ZCCHC4 is a newly identified m6A RNA methyltransferase and is highly conserved in multicellular organisms. ZCCHC4-mediated m6A4220 methylation in 28S rRNA promotes ribosome assembly and translation, which in turn impacts cell proliferation and tumor growth. Distinct from what was observed for all other m6A methyltransferases, ZCCHC4 is organized into four domains, with three flanking zinc finger domains packed around the MTase domain, forming an integrated RNA-binding platform. Through structural, biochemical, and enzymatic characterization of ZCCHC4, a recently reported rRNA m6A writer, this study reveals the molecular basis for the ZCCHC4-mediated m6A4220 modification of 28S rRNA.

The crystal structure of ZCCHC424-464, in complex with S-adenosyl-L-homocysteine (SAH), product of methyl donor S-adenosyl-L-methionine (SAM), was refined to 3.1 Å resolution. There are six ZCCHC424-464 complexes in one asymmetric unit; among these, two ZCCHC4 molecules engage swapping of the N-terminal tail (residues M26-V28) of one to pair in antiparallel with residues F48-V51 of the other, likely due to crystal packing effects. The structure of ZCCHC424-464 reveals four closely packed domains: an N-terminal GRF zinc finger domain is followed by a C2H2 zinc finger domain, an MTase domain, and a C-terminal CCHC zinc finger domain, folded into an integrated structural unit. The SAH molecule snugly fits into a fully closed pocket, lined by a loop connecting the C2H2 domain and the MTase domain (cofactor loop: residues P163-F175), the terminal ends of αG-helix and β8-strand, and the DPPF (D276-P277-P278-F279) catalytic motif. The homocysteine moiety of SAH is surrounded by the side chains of L174-F175, T200-R202, and D276, with the amino group donating a hydrogen bond to the side-chain carboxylate of D276 and the carboxylate receiving a hydrogen bond from the backbone amide of F175. On the other end, the adenosyl moiety of SAH is embraced by the side chains of I226, N243, M244, and F245 through van der Waals contacts, with the N6 atom further forming a hydrogen bond with the side-chain carbonyl group of N243. Astonishingly, structural comparison of ZCCHC4 with METTL16, as well as other RNA methyltransferases, also reveals a striking difference in the active-site conformation: the D/N-P-P-F/W catalytic motifs of METTL16, METTL3, METTL5, and CAPAM are all readily accessible for RNA contacts; in contrast, the corresponding DPPF motif in ZCCHC4 is shielded from solvent exposure by the loop connecting αK and β13 (hereafter referred to as regulatory loop), which wedges into the catalytic center for interaction with the active-site residues. Of particular note, residue D276 forms a bifurcated side-chain hydrogen bond with regulatory loop residue Y340, which potentially occludes D276 from nucleophilic attack during the methylation reaction.

>[6x]SGMEVVLPLDPAVPAPLCPHGPTLLFVKVTQGAAATRRFYACSACRDRKDCNFFQWEDEKLSGARLAAREAHNRRCQPPLSRTQCVERYLKFIELPLTQRKFCQTCQQLLLPDDWGQHSEHQVLGNVSITQLRRPSQLLYPLENAATNAQYLFADRSCQFLVDLLSALGFRRVLCVGTPRLHELIKLTASGDKKSNIKSLLLDIDFRYSQFYMEDSFCHYNMFNHHFFDGKTALEVCRAFLQEDKGEGIIMVTDPPFGGLVEPLAITFKKLIAMWKEGQSQDDSHKELPIFWIFPYFFESRICQFFPSFQMLDYQVDYDNHALYKHGKTGRKQSPVRIFTNIPPNKIILPTEEGYRFCSPCQRYVSLENQHCELCNSCTSKDGRKWNHCFLCKKCVKPSWIHCSICNHCAVPDHSCEGPKHGCFICGELDHKRSTCPNIATS>MQTKKNEIWVGIFLLAALLAALFVCLKAANVTSIRTEPTYTLYATFDNIGGLKARSPVSIGGVVVGRVADITLDPKTYLPRVTLEIEQRYNHIPDTSSLSIRTSGLLGEQYLALNVGFEDPELGTAILKDGDTIQDTKSAMVLEDLIGQFLYGSKGDDNKNSGDAPAAAPGNNETTEPVGTTK[6x];> MFKRLMMVALLVIAPLSAATAADQTNPYKLMDEAAQKTFDRLKNEQPQIRANPDYLRTIVDQELLPYVQVKYAGALVLGQYYKSATPAQREAYFAAFREYLKQAYGQALAMYHGQTYQIAPEQPLGDKTIVPIRVTIIDPNGRPPVRLDFQWRKNSQTGNWQAYDMIAEGVSMITTKQNEWGTLLRTKGIDGLTAQLKSISQQKITLEEKK

The Maintenance of Lipid Asymmetry (Mla) pathway is a multicomponent system found in all gram-negative bacteria that contributes to virulence, vesicle blebbing and preservation of the outer membrane barrier function. The pathway consists of an OM lipoprotein component (MlaA), found as part of a complex with either OmpC or OmpF7,8; a periplasmic GPL chaperone (MlaC) which shuttles GPL across the periplasm; and an IM ATP binding cassette (ABC) transporter complex (MlaFEDB). MlaFEDB consists of four proteins: MlaE an ABC permease protein; MlaD a membrane anchored MCE (mammalian cell entry) domain containing protein forming a homo-hexameric ring that faces the periplasm; MlaF, an ABC ATPase; and MlaB, a STAS (Sulfate Transporter and Anti-Sigma factor antagonist) domain protein proposed to have a regulatory function. Specifically, we report the structure of E. coli MlaC in complex with the MlaD hexamer, in two different stoichiometries (1:6 and 2:6, respectively), stabilised through the binding of cardiolipin.

Masked refinement and 3D classification, focusing on one MlaD hexamer, revealed two distinct species, one with a single MlaC bound to a MlaD32-183 hexamer, and another with two MlaC molecules bound, with final resolutions of 4.35 Å and 4.38 Å, respectively. In the MlaCD(1:6) structure, a single copy of MlaC is bound offset from the central cavity, on top of the main MlaD ring, predominantly interacting with a single MlaD32-183 monomer (henceforth termed MlaD1) but making additional interactions between both the clockwise (MlaD2) and counter-clockwise MlaD32-183 (MlaD6) subunits. MlaCD(1:6) has a Cɑ RMSD of between 0.7 and 0.8 Å in the core fold across all pairwise protomer alignments. In the case of MlaCD(1:6) binding clearly results in the 6-fold symmetry of the MlaD hexamer being broken, as evidenced by changes in the angles between MlaD monomers. Interestingly, the largest deviations occur distal from MlaC binding, for example between MlaD monomers 2, 3 and 4. Importantly, such a break in symmetry was not observed in the structures of MlaD within the MlaFEDB inner-membrane assembly, and is therefore possibly not representative of the physiological binding event. Whilst MlaC Pro124, does not make any observed close contacts in our structure, however, based on its position, the most likely location for interaction would be with the β6-β7 loop of MlaD2. However, many ABC transporters have been shown to have an asymmetric mechanism, suggesting the binding of a single MlaC monomer could also be feasible. The presence of two GPLs within the central binding pocket and a single MlaC bound can be reconciled by both GPLs binding to a single MlaC monomer.> MVVLDKKLLERLTSRKVPLEQLEDMEKRCFLSTFTYQDAFDLGTYIRNAVKENFPEKPVAIDISLPNGHCLFRTVTYGGSALDN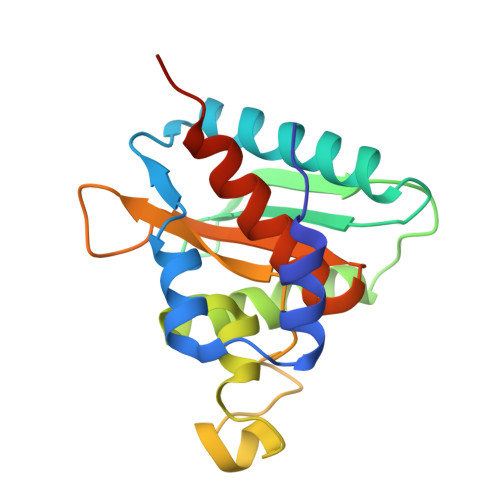DFWIQRKKKTALRFGHSSFYMGCKKGDKTPEEKFFVDSKEYAFHGGAVLIQSERSDYPYACLTISGLKQEEDHLMAVSSLIAFANESLEEDLNLD> GFPTELKPGTNQFLTTDDGTSPPILPGFEPTPLIHIPGEFTSLLDLCQIETILEVNNTTGTIGVSRLLIPVRAQNNVDQLCASFQVDPGRNGPWQSTMVGQICRYYTQWSGSLKVTFMFTGSFMATGKMLIAYTPPGSAQPATREAAMLGTHIVWDFGLQSSVTLVIPWISNTHFRAVKIGGVYDYYATGIVTIW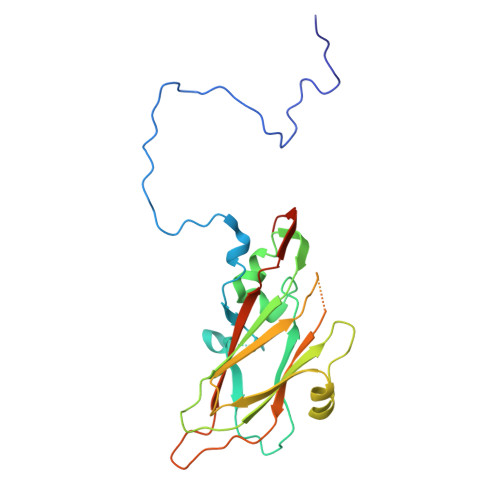YQTNFVVPPDTPTEANIIALGAAQKNFTLKLCKDTDEIQQTAAYQ>GSHMTYVILPLEMKKGRGYVYQLEYHLIWCVKYRHQVLVGEVADGLKDILRDIAAQNGLEVITMEVMPDHVHLLLSATPQQAIPDFV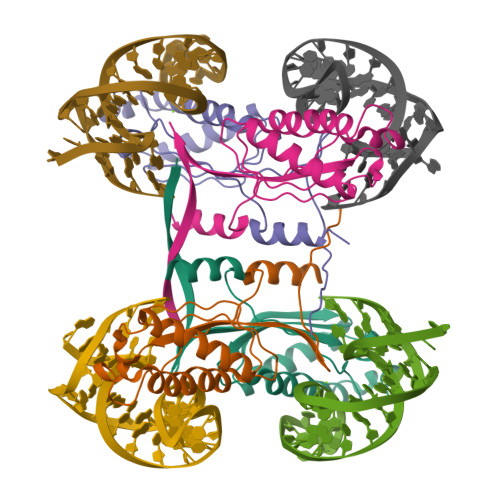KALKGASARRMFVAYPQLKEKLWGGNLWNPSYCILTVSENTRAQIQKYIESQHDKE[4x]> SFPVQILPNLYLGSARDSANLESLAKLGIRYILNVTPNLPNFFEKNGDFHYKQIPISDHWSQNLSRFFPEAIEFIDEALSQNCGVLVHC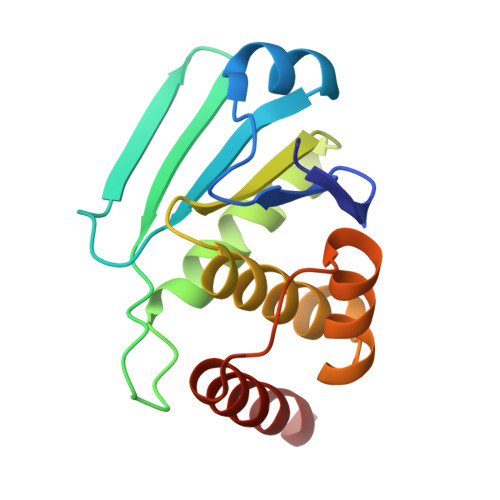LAGVSRSVTVTVAYLMQKLHLSLNDAYDLVKRKKSNISPNFNFMGQLLDFERSLRLE>[9x]MGLEAVRKRPGMYIGSTDSRGLHHLVYEIVDNAVDEALSGYGNEINVTIQKDNSICVADSGRGMPTGMHASGIPTVEVIFTVLHAGGKFGQGG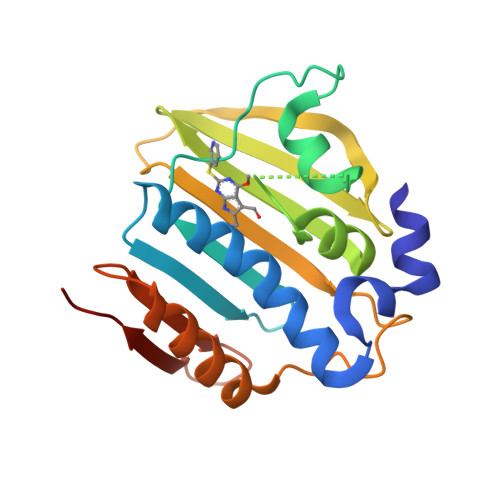YKTSGGLHGVGASVVNALSKWLEVHIVRDGVEYMERFEDGGKPVGTLKKIGKTKKRNGTSVTFLPDDTIFSTTNFSYEILAERLRESAFLLKGVKITLTDERGEEPKEEVFHYEELEHHHHHH> MVGAGAYAYKTMKEDEKRYNERISGLGLTPEQKQKKAALSASEGEEVPQDKAPSHVPFLLIGGGTAAFAAARSIRARDPGARVLIVSEDPELPYMRPPLSKELWFSDDPNVTKTLRFKQWNGKERSIYFQPPSFYVSAQDLPHIENGGVAVLTGKKVVQLDVRDNMVKLNDGSQITYEKCLIATGGTPRSLSAIDRAGAEVKSRTTLFRKIGDFRSLEKISREVKSITIIGGGFLGSELACALGRKARALGT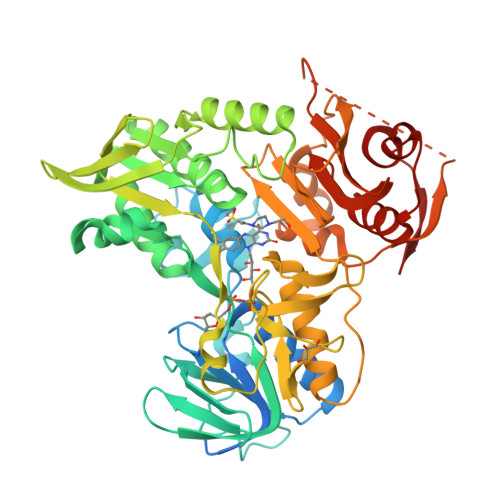EVIQLFPEKGNMGKILPEYLSNWTMEKVRREGVKVMPNAIVQSVGVSSGKLLIKLKDGRKVETDHIVAAVGLEPNVELAKTGGLAIDSDFGGFAVNAELQAASNIWVAGDAACFYDIKLGRRRVEHHDHAVVSGRLAGENMTGAAKPYWHQSMFWSDLGPDVGYEAIGLVDSSLPTVGVFAKATAQDNPKSATEQSGTGIRSESETESEASEITIPPSTPAVPQAPVQGEDYGKGVIFYLRDKVVVGIVLWNIFNRMPIARKIIKDGEQHEDLNEVAKLFNIHEDLEVLFQ>MKKWSHPQFEKGGSDYKDDDDKPICTIHEHDRVSADRGGDSPHTTHALVDRLMAGEPYAVAFGGQGSAWLETLEELVSATGIETELATLVGEAELLLDPVTDELIVVRPIGFEPLQWVRALAAEDPVPSDKHLTSAAVSVPGVLLTQIAATRALARQGMDLVATPPVAMAGHSQGVLAVEALKAGGARDVELFALAQLIGAAGTLVARRRGISVLGDRPPMVSVTNADPERIGRLLDEFAQDVRTVLPPVLSIRNGRRAVVITGTPEQLSRFELYCRQISEKEEADRKNKVRGGDVFSPVFEPVQVEVGFHTPRLSDGIDIVAGWAEKAGLDVALARELADAILIRKVDWVDEITRVHAAGARWILDLGPGDILTRLTAPVIRGLGIGIVPAATRGGQRNLFTVGATPEVARAWSSYAPTVVRLPDGRVKLSTKFTRLTGRSPILLAGMTPTTVDAKIVAAAANAGHWAELAGGGQVTEEIFGNRIEQMAGLLEPGRTYQFNALFLDPYLWKLQVGGKRLVQKARQSGAAIDGVVISAGIPDLDEAVELIDELGDIGISHVVFKPGTIEQIRSVIRIATEVPTKPVIMHVEGGRAGGHHSWEDLDDLLLATYSELRSRANITVCVGGGIGTPRRAAEYLSGRWAQAYGFPLMPIDGILVGTAAMATKESTTSPSVKRMLVDTQGTDQWISAGKAQGGMASSRSQLGADIHEIDNSASRCGRLLDEVAGDAEAVAERRDEIIAAMAKTAKPYFGDVADMTYLQWLRRYVELAIGEGNSTADTASVGSPWLADTWRDRFEQMLQRAEARLHPQDFGPIQTLFTDAGLLDNPQQAIAALLARYPDAETVQLHPADVPFFVTLCKTLGKPVNFVPVIDQ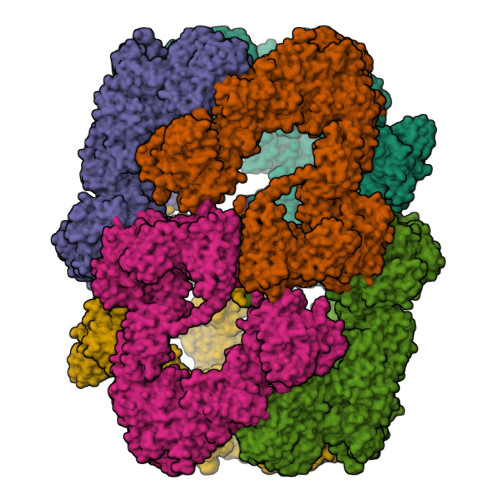DVRRWWRSDSLWQAHDARYDADAVCIIPGTASVAGITRMDEPVGELLDRFEQAAIDEVLGAGVEPKDVASRRLGRADVAGPLAVVLDAPDVRWAGRTVTNPVHRIADPAEWQVHDGPENPRATHSSTGARLQTHGDDVALSVPVSGTWVDIRFTLPANTVDGGTPVIATEDATSAMRTVLAIAAGVDSPEFLPAVANGTATLTVDWHPERVADHTGVTATFGEPLAPSLTNVPDALVGPCWPAVFAAIGSAVTDTGEPVVEGLLSLVHLDHAARVVGQLPTVPAQLTVTATAANATDTDMGRVVPVSVVVTGADGAVIATLEERFAILGRTGSAELADPARAGGAVSANATDTPRRRRRDVTITAPVDMRPFAVVSGDHNPIHTDRAAALLAGLESPIVHGMWLSAAAQHAVTATDGQARPPARLVGWTARFLGMVRPGDEVDFRVERVGIDQGAEIVDVAARVGSDLVMSASARLAAPKTVYAFPGQGIQHKGMGMEVRARSKAARKVWDTADKFTRDTLGFSVLHVVRDNPTSIIASGVHYHHPDGVLYLTQFTQVAMATVAAAQVAEMREQGAFVEGAIACGHSVGEYTALACVTGIYQLEALLEMVFHRGSKMHDIVPRDELGRSNYRLAAIRPSQIDLDDADVPAFVAGIAESTGEFLEIVNFNLRGSQYAIAGTVRGLEALEAEVERRRELTGGRRSFILVPGIDVPFHSRVLRVGVAEFRRSLDRVMPRDADPDLIIGRYIPNLVPRLFTLDRDFIQEIRDLVPAEPLDEILADYDTWLRERPREMARTVFIELLAWQFASPVRWIETQDLLFIEEAAGGLGVERFVEIGVKSSPTVAGLATNTLKLPEYAHSTVEVLNAERDAAVLFATDTDPEPEPEEDEPVAESPAPDVVSEAAPVAPAASSAGPRPDDLVFDAADATLALIALSAKMRIDQIEELDSIESITDGASSRRNQLLVDLGSELNLGAIDGAAESDLAGLRSQVTKLARTYKPYGPVLSDAINDQLRTVLGPSGKRPGAIAERVKKTWELGEGWAKHVTVEVALGTREGSSVRGGAMGHLHEGALADAASVDKVIDAAVASVAARQGVSVALPSAGSGGGATIDAAALSEFTDQITGREGVLASAARLVLGQLGLDDPVNALPAAPDSELIDLVTAELGADWPRLVAPVFDPKKAVVFDDRWASAREDLVKLWLTDEGDIDADWPRLAERFEGAGHVVATQATWWQGKSLAAGRQIHASLYGRIAAGAENPEPGRYGGEVAVVTGASKGSIAASVVARLLDGGATVIATTSKLDEERLAFYRTLYRDHARYGAALWLVAANMASYSDVDALVEWIGTEQTESLGPQSIHIKDAQTPTLLFPFAAPRVVGDLSEAGSRAEMEMKVLLWAVQRLIGGLSTIGAERDIASRLHVVLPGSPNRGMFGGDGAYGEAKSALDAVVSRWHAESSWAARVSLAHALIGWTRGTGLMGHNDAIVAAVEEAGVTTYSTDEMAALLLDLCDAESKVAAARSPIKADLTGGLAEANLDMAELAAKAREQMSAAAAVDEDAEAPGAIAALPSPPRGFTPAPPPQWDDLDVDPADLVVIVGGAEIGPYGSSRTRFEMEVENELSAAGVLELAWTTGLIRWEDDPQPGWYDTESGEMVDESELVQRYHDAVVQRVGIREFVDDGAIDPDHASPLLVSVFLEKDFAFVVSSEADARAFVEFDPEHTVIRPVPDSTDWQVIRKAGTEIRVPRKTKLSRVVGGQIPTGFDPTVWGISADMAGSIDRLAVWNMVATVDAFLSSGFSPAEVMRYVHPSLVANTQGTGMGGGTSMQTMYHGNLLGRNKPNDIFQEVLPNIIAAHVVQSYVGSYGAMIHPVAACATAAVSVEEGVDKIRLGKAQLVVAGGLDDLTLEGIIGFGDMAATADTSMMCGRGIHDSKFSRPNDRRRLGFVEAQGGGTILLARGDLALRMGLPVLAVVAFAQSFGDGVHTSIPAPGLGALGAGRGGKDSPLARALAKLGVAADDVAVISKHDTSTLANDPNETELHERLADALGRSEGAPLFVVSQKSLTGHAKGGAAVFQMMGLCQILRDGVIPPNRSLDCVDDELAGSAHFVWVRDTLRLGGKFPLKAGMLTSLGFGHVSGLVALVHPQAFIASLDPAQRADYQRRADARLLAGQRRLASAIAGGAPMYQRPGDRRFDHHAPERPQEASMLLNPAARLGDGEAYI[6x]> MTSVTRSEIIDEKGPVMSKTHDHQLESSLSPVEVFA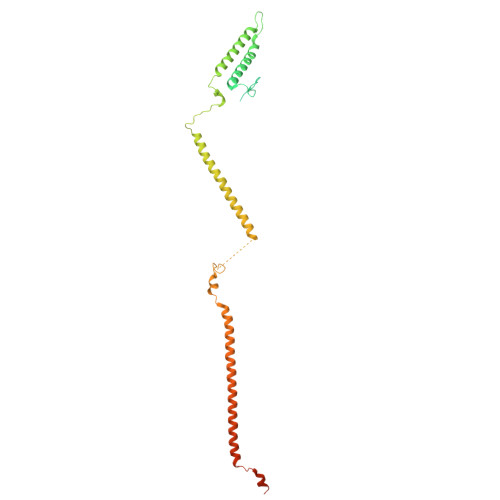KTSASLEMNQGVSEERIHLGSSPKKGGNCDLSHQERLQSKSLHLSPQEQSASYQDRRQSWRRASMKETNRRKSLHPIHQGITELSRSISVDLAESKRLGCLLLSSFQFSIQKLEPFLRDTKGFSLESFRAKASSLSEELKHFADGLETDGTLQKCFEDSNGKASDFSLEASVAEMKEYITKFSLERQTWDQLLLHYQQEAKEILSRGSTEAKITEVKVEPMTYLGSSQNEVLNTKPDYQKILQNQSKVFDCMELVMDELQGSVKQLQAFMDESTQCFQKVSVQLGKRSMQQLDPSPARKLLKLQLQNPPAIHGSGSGSCQHHHHHH>[2x]VTGDTDQPIHIESDQQSLDMQGNVVTFTGNVIVTQGTIKINADKVVVTRPGGEQGKEVIDGYGKPATFYQMQDNGKPVEGHAS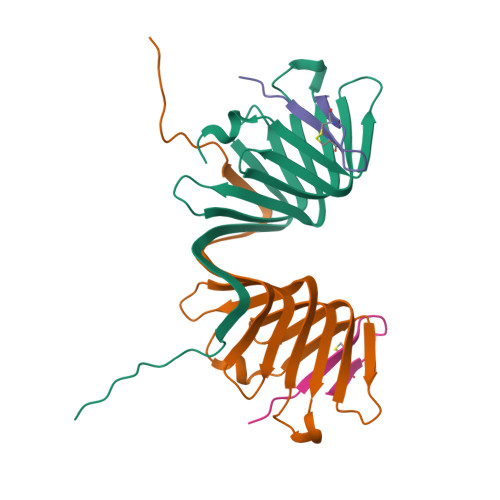QMHYELAKDFVVLTGNAYLQQVDSNIKGDKITYLVKEQKMQAFSDKGKR;>GSKPVPIIACNRKTGKCRRI[2x]>GDTASLLVENGRGNTLWPQVVSVLQAKNYTITQRDDAGQTLTTDWVQWNRLD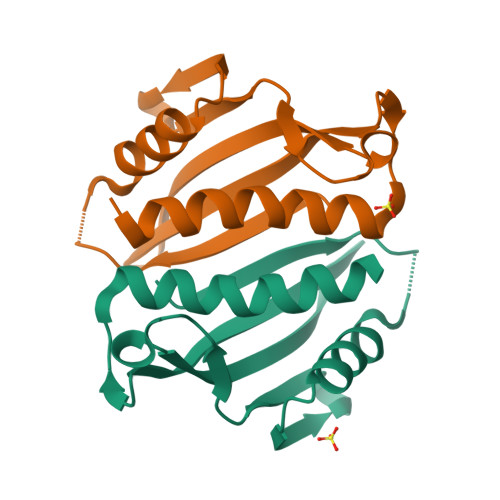EDEQYRGRYQISVKPQGYQQAVTVKLLNLEQAGKPVADAASMQRYSTEMMNVISAGLDKS[4x]>[2x]ACYCRIPACIAGER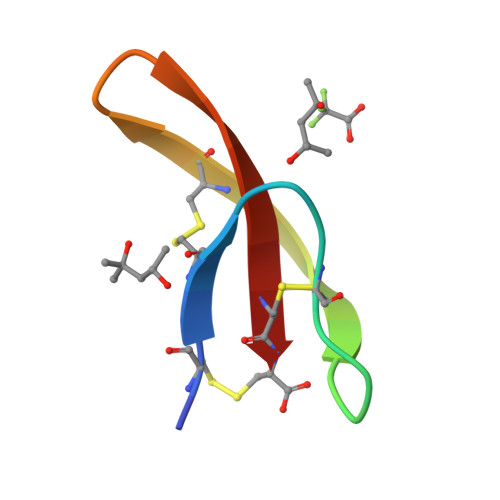RYGTCIAQGRLWAFCC> QGSPTQWYDSITGVTFSRFYQQDTDASWGYIFPSASGGQAPDEFIGLFQGPASAGWIGNSLGGSMRNNPLLVGWVDGSTPRISARWATDYAPPSIYSGPRLTILGSSGTNGNIQRIVYRCQNCTRWTGGAGGIPTTGSAVFGWAFHSTTKPLTPSDPSSGLYRHSHAAQYGFDI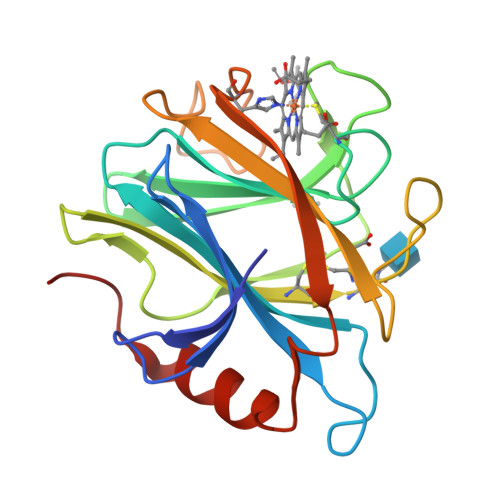GNARTTLYDYYLQQLTNAPPLSG>[8x]DD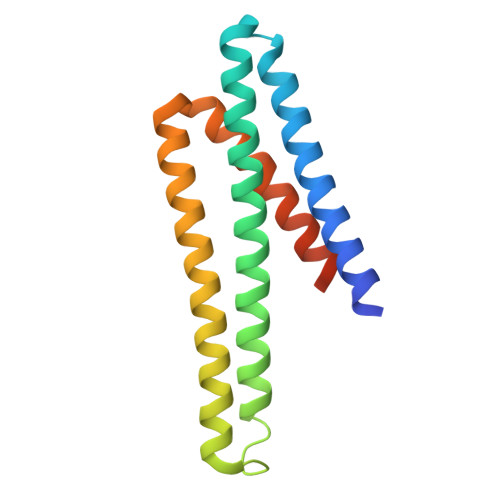SRISSALQNLWTAAQAAMAAAVKAKAAEIAATKTPEEAKKVAEIAEKAIEIGKLAADAALGIAAAAGGKAVIAKMADGISPEKQAKYLAKFDAEAAAAKEGLAEAEKILKELLKEDPEAAKALTATALAAAAAAIAALLAAGLEHHHHHH> VYFLKKKKNKILTIALVASLAASVSFGSVLYYSFSDNHISFDTSSNGITDAELAPINNAINDAIVSNRDNKLKPSEEKIIKETEKKIEEKIIIPPAKKEEKIEAAKPIPKPVVRKPETKITSPKITRRKQTITIAGIEVEAEIEGPPGFVTHQRDKDRKISNPTKPYQNHTVNKILSVKVTDKLKEQVAKDALSGGNGYDEGVGLFNNSIFNVFKEEFNSGKELNDILSSLESVARQNSGAFQNTLERYKKMLDSNNVINFLKSEAQKEYPKLKSKFQTKNQEYIWLIANLDQSKFTKIASTSEKYLEKGLTISPRSAFINEAGEIDSNGWGPPDEYNTVTSRLRRDNSEYRVFDYDEYYSRSSDRIANGTYPGWVKEDVSEPYSKKYNFKASDGIRFSKLERINPNPAKGKLNSGLVLDLDVSNDEAYRRSKELIEKLQKDGEQITSYRIKNMGEKNSDQAFKDILGALPKDIQQLELFFSDKATNTASLIALENKNIKELSLYTSGNSLKKAWSYNPLALRNTTWINTIDYNVSAEYSSHDKITTRITFNTLAFDQEDFSNGSYERINDGLRMVYYARNNEPFFQGGHGPGLEPDKKLGQNSYPTGLDFSRVTGIKSLKGLRFDDDLDTSNEPRKITELTLYNNESYFEISSDELNEANLQHLSTGEGNPEKPKIHFSNGNNTTSIRISGKTLLSDEGRRNLDKYFEYNESLRNSGKQIQIPNGSD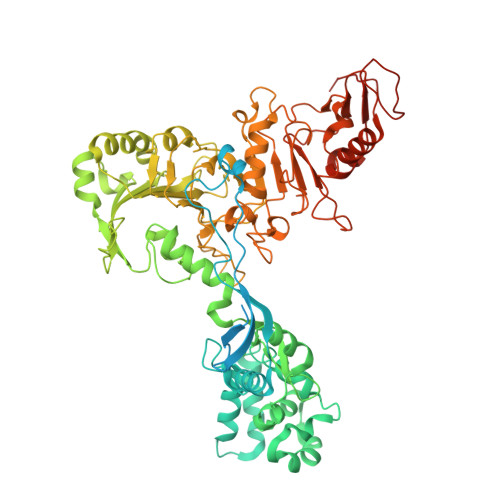ELKKQLEGWGYKVSTASDRSFT> MTVRKNQATLTADEKRRFVAAVLELKRSGRYDEFVRTHNEFIMSDTDSGERTGHRSPSFLPWHRRFLLDFEQALQSVDSSVTLPYWDWSADRTVRASLWAPDFLGGTGRSTDGRVMDGPFAASTGNWPINVRVDSRTYLRRSLGGSVAELPTRAEVESVLAISAYDLPPYNSASEGFRNHL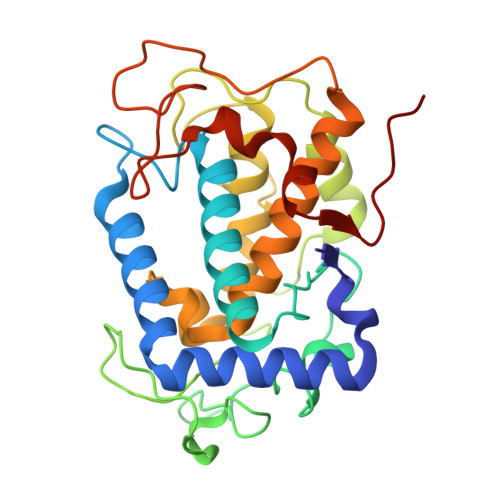EGWRGVNLHGRVHVWVGGQMATGVSPNDPVFWLHHAYVDKLWAEWQRRHPDSAYVPTGGTPDVVDLNETMKPWNTVRPADLLDHTAYYTFDALEHHHHHH>GSDSGTLNYEVYKYNTNDTSIANDYFNKPAKYIKKNGKLYVQITVNHSHWITGMSIEGHKENIISKNTAKDERTSEFEVSKLNGKIDGKIDVYIDEKVNGKPFKYDHHYNITYKFNGPTDVAGANAPG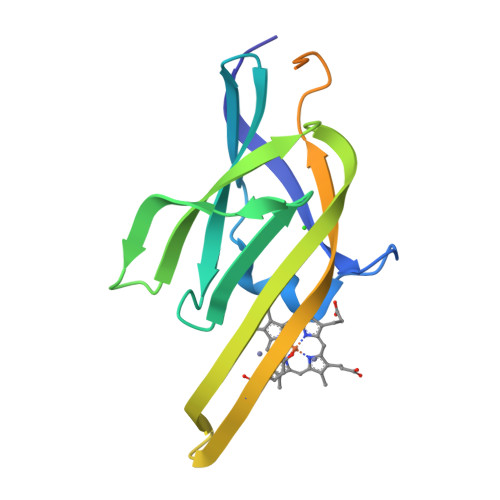KDDKNSASGSDKGSDGTTTGQSESNSSNKDKVE[2x]>MAHHHHHHMSNQRVNKRVVITGLGLVTPVGLNVNSSWKNIVDGVSGIKTITEFDTSKLACKIAGLIDNSEKDGFKLENFTQADDINRLSKMDKFIHYGVAAATEAVEDSGWLPDDEKSRDRTGLILGSGIGGLKMIEDTSIKLYQENNGKVSPFFIPASLINLLSGLVSIKYGFSGPNQTAVTACSTGAHAIGDAMRMIKHGYADVMIAGGAEAPVTPVGVAGFVAARALCTKYNDNPKKASRPWDKDRSGFVMGEGAGVVVLEEYEHALNRGAKVYGEVIGYGSTGDAYHMTAPHPEGRGAYRAMRDAMLDATITPDMIDYINAHGTSTTLGDGIELAAVQKLFLEANPKVLMSSTKSSIGHLLGAAGSVEFIFSALAIRDQIAPPTLNLDTPMDEVNIDLVALKAKKTKIDYVL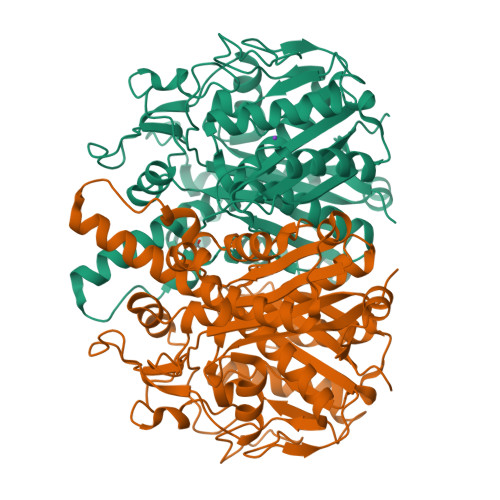SNSFGFGGTNASLVIKSILVK[2x]>[3x]SNAMKVSGWGEMVKVVATNKKAYTDYEILETYEAGIVLTGTE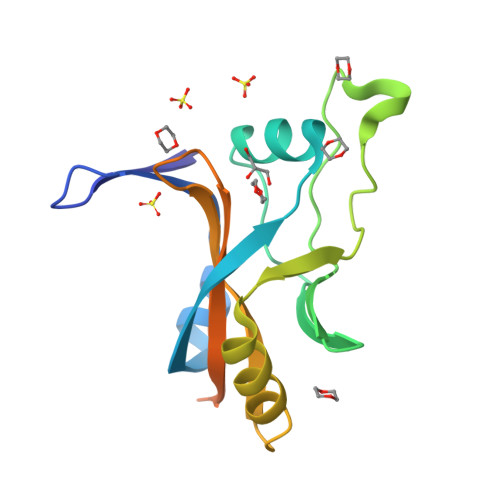VKSLRNGSVNFKDSFCRFKNGELYLLNLHIPPYSHGGVYNHDPERPRKLLLHKRELKRLMGKVQEEGVTIVPLKIYFNDRGIAKVEIAVARGKKKYDKREAIKKREMERKIREYMKYSR>DINGGGATLPQKLYLTPDVLTAGFAPYIGVGSGKGKIAFLENKYNQFGTDTTKNVHWAGSDSKLTATELATYAADKEPGWGKLIQVPSVATSVAIPFRKAGANAVDLSVKELCGVFSGRIADWSGITGAGRSGPIQVVYRAESSGTTELFTRFLNAKCTTEPGTFAVTTTFANSYSLGLTPLAGAVAATGSDGVMAALNDTTVAEGRITYMSPDFAAPTLAGLDDATKVARVGKGVVNGVAVEGKSPAAANVSAAISVVPLPAAADRGNPDVWVPVFGATTGGGVVAYPDSGYPILGFTNLIFSQCYANATQTGQVRDFFTKHYGTSANNDAAIEANAFVPLPSNWKAAVRASFLTASNALSIGNTNVCNGKGRPQ[2x]

DING is a family of proteins with molecular mass of approximately 40 kDa, with a conserved N-terminal sequence of DINGGG. DING proteins are one of three families within a superfamily of bacterial phosphate-binding proteins. To date, the crystal structures of two DING proteins, i.e. human phosphate-binding protein (HPBP) and DING protein from Pseudomonas fluorescens SBW25 (PflDING), have been reported. In both structures, a phosphate ion was captured in a binding cleft between two domains.

To enable further study of DING proteins, an E. coli expression system for HPBP was constructed. Then, the insoluble rHPBP was unfolded with 6 M guanidinium hydrochloride and 1 mM β-mercapto­ethanol. The chemically unfolded rHPBP was refolded by the dilution method. The refolded rHPBP was further purified by chromatography, and the final yield was 43 mg per litre of culture. To evaluate whether rHPBP was refolded correctly, the purified rHPBP was crystallized and its structure was determined. The structure of rHPBP was determined at a resolution of 1.03 Å. The revealed structure was well superposed on the native HPBP with r.m.s.d. of 0.04 Å for 327 Cα atoms. A phosphate ion was captured at the identical site to native HPBP, with identical residues participating in recognition. Furthermore, two disulfide bonds were formed correctly. Based on these observations, it was concluded that rHPBP was correctly refolded to the native structure.> MAFRGSSARLAATPGVGIAPETTPVKYVPEMLNIQNAKWWNGRGKPVYRSTYNEKSWLEKARWGAFTKGSRPVMRQRYSAAALKEALEMVPEGFETCDVPRPPQRIRAQSEGVVGRWYTNYWTLHSVRYQCQLAGVEWQFGERQRPRTNYDEPHMYTDFEETKAIRDYRSRWINVNRSLVGMSRRMKESEEEAR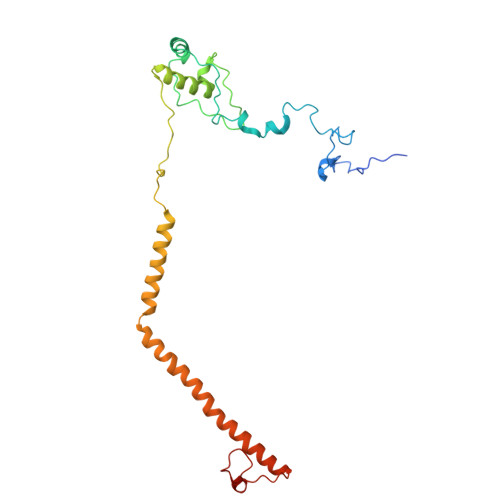YLHFKKVQDTFWSNRKVLVNRIKSMHNQGTLQSAKDLPIKTINIKAFLAE> MKQYLELMQKVLDEGTQKNDRTGTGTLSIFGHQMRFNLQDGFPLVTTQRCHLRSIIHELLWFLQGDTNIAYLHENNVTIWDEWADENGDLGPVYGKQWRAWPTPDGRHIDQITTVLNQLKNDPDSRRIIVSAWNVGELDKMALAPCHAFFQFYVADGKLSCQLYQRSCDVFLGLPFNIASYALLVHMMAQQCDLEVGDFVWTGGDTHLYSNHMDQTHLQLSREPRPLPKLIIKRKPESIFDYRFEDFEIEGYDPHPGIKAPV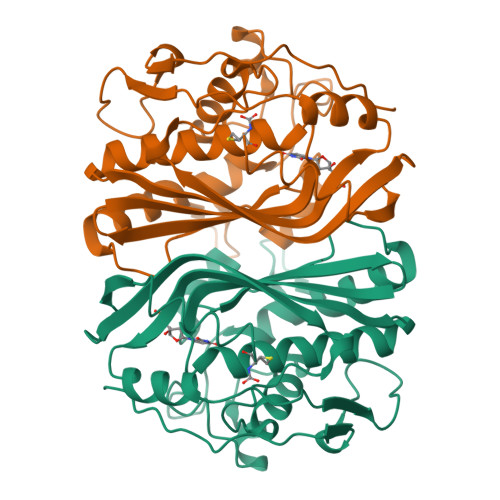AI CydDC is a prokaryotic ATP-binding cassette (ABC) transporter required for heme assembling in respiratory cytochrome bd oxidase, a promising target for drug discovery. In our structures, CydC and CydD form a heterodimer with each subunit composed of one transmembrane domain (TMD) and one nucleotide-binding domain (NBD). TM4 and TM5 of one subunit associate with TM1-3 and TM6 of another to form a helix bundle in a “domain swapping” manner. The overall fold of CydDC belongs to the type IV family of ABC transporters, commonly known as exporters.

In the NBD of MsCydC, half of the Linking Loop, the β1 strand, and the A-loop are missing. The rest of the Linking Loop then connects directly with β2, forming a new “Linking-β2 Loop” which passes through the front side of NBD and covers the ATP-binding site. Arg324 and Arg326 in the Linking-β2 Loop play an important role in stabilizing ATP by sandwiching its adenosine ring. In the NBD of MsCydD, the β1–β2 hairpin becomes really short by deleting a fragment containing the A-loop, so that the distance between the adenosine group of ATP and the tip of hairpin (Ala315) is 21 Å. To rescue the function of NBD, the adenosine ring of ATP is stabilized by the sidechain of Arg85 from ICL1 located between TM2 and TM3. At the periplasmic side of TMDs, there are significant shifts for the TM helices in the outward-facing state of MsCydDC. The TM3–TM4 pair, TM5–TM6 pair and TM1 of MsCydC all move away from the center of the helix bundle. Thus, the central cavity opens towards the periplasm and gaps are created between TM1C and TM6C, and between TM5C and TM2D. In the ATP-bound structures, the two axial His residues are 12.9 Å far away from each other in MsCydDC (or 12.7 Å in EcCydDC).

>[2x]LRHDPLLRLTLELLRPRLGRFLLAAALGVLSLGSALALAGISAWLITRAWQMPPVLDLTVAVVAVRALGISRGVLGYCQRLASHDSALRAAANARTGLYRKLADAPPDEAMRLPSGELVARLGPAVDELADVLVRALLPIVVAVVLGCAAVGVIAVISPASAAVLAVCLVVAGVVAPALAARAAHASETVAAEHRSQRDTAGMLALEHAPELRVSGRLDSVIATFERHHRAWGEAADRAAAPAAVAAAMPTAAMGVSVVGAVIAGIALAPTVAPTTAAILMLLPLSAFEATTALPDAAAQLMRSRVAARRLLELTTPTPLRSRPDVATVDLAPGDRLAVVGPSGSGKTTMLMAIADRLNGAGGETPQRAAVFAEDAHLFDTTVRDNLLVVRGDATDTELVAALDRVGLGEWLAGLPDGLSTVLVGGAAAVSAGQRRRLLIARALISAFPVVLLDQPTENLDAGDARQMLEGLLTPGALFAADRTVVVATHHLPPGFDCPIVRCT;>[2x]SYFQSNVVIAGCTIASAVVLAHIVAGIITNPATALGGETDWAPGLVALAVLWSVRVVAQWFQGRLSQRGATAVIGELSRQVLSSVTTSSPRRLAADRDSAAAVVTRGLDGLRPYFTGYLPAVVLAGILTPAALVVMAAYDWQAAAIVVIALPLIPIFMVLIGLLTAERSAAALTAMTTLQGRMLDLIAGIPTLRAVGRAGGSVQRIAELSASHRRSTMATLRISFLSALVLELLATLGVALVAVSVGLRLVFGDMTLAAGLTALLLAPEVFWPLRRVGAAFHAAQDGKTAAEQALRLCAEPHPPTGHEVVPAGAPVIEVPALKAVMEPGRVTVLTGPNGVGKSTLLQAILGLQESPCGPILVAGVEVGALDRSAWWGRLAWMPHRPVLVPGTVRENLELLGPVPGLDEVCRSVGFDEVLGELPDGSETPLGRGGVGLSLGQRQRLGLVRALGAPADVLLLDQPTAHLDGALEDRVLAAIVARARAGATVVMVGHRAPVLAAADHVVTMESSLVAP>[4x]EVKLILYHWTHSFSSQKVRLVIAEKALKCEEHDVSLPLSEHNEPWFMRLNSTGEVPVLIHGENIICEATQIIDYLEQTFLDERTPRLMPDKESMYYPRVQHYRELLDSLPMDAYTHGCILHPELTVDSMIPAYATTRIRSQIGNTESELKKLAEENPDLQEAYIAKQKRLKSKLLDHDNVKYLK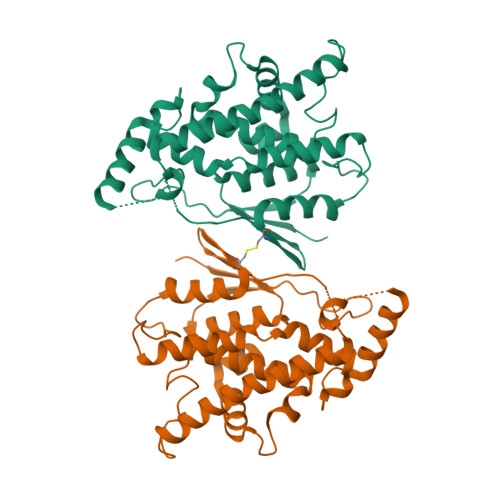KILDELEKVLDQVETELQRRNEETPEEGQQPWLCGESFTLADVSLAVTLHRLKFLGFARRNWGNGKRPNLETYYERVLKRKTFNKVLG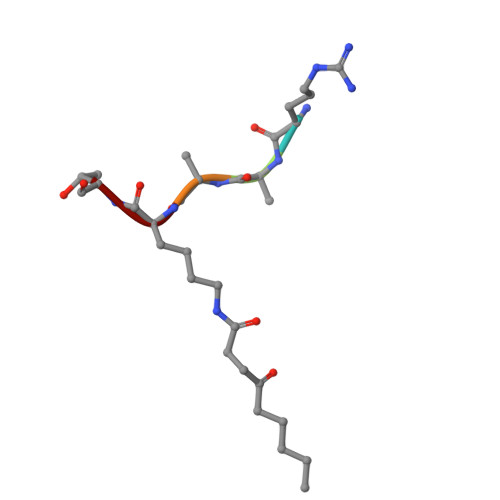> RAAKT>MSQEQLTGSSILAKSLKSLGVDVIFGIVGVPVVEVAEACIAEGIRFIGCRNEQSASFAAGAWGYLNKRPGVCLTVSGPGVVNAISGLYNAQANCWPMILIGGSCETNQIGMGAFQELDQVDACRNYTKFSGKCADLETIPFIVNKAYQVSKAGRPGPTYVDLPADLIQATTSKLPKLPEPFETPYCLPHTKDLSAAIEILKNSKRPLLVVGKGATYSRCENELKALVEEFNVPFLPTPMAKGILPDNHSLNAGSARSLALRKADVIVLLGARLNWMMQFGNRLNPQTKIIHVDISPEEFNINKKIDIGLFGNIPETIELIHQGLKKSGKSYSWIHFKNELQPNIEKNQEKLQKFLTAPLSPLMNHQQALNTVEEVLSKQFNGDYFLVSEGARTMDVTRMLVSSHLPRRRLDAGTLGVMGIGLGYALAGQLTHPDKKVVAIMGDSAFGFSAMEIETAARCKLPLIIIIINNNGIYHGLDDIKSVPSDKLPSFTLMPETRYDLLANSVYGQGFLVKDSTQLQSALQKCFNFDGVSIVNVMIDHRPASEGLYWLTREFSPAGQSKL[4x]

One such enzyme is 2-hydroxyacyl-CoA lyase/synthase (HACL/S), which catalyzes the reversible cleavage of 2-hydroxyacyl-CoA (2hcCoA) into formyl-CoA (fCoA) and an aldehyde or ketone. Originally identified in the mammalian α-oxidation pathway of 3-methyl-branched fatty acids, HACL/S has demonstrated remarkable catalytic reversibility, as it is capable of condensing fCoA with various substrates covering a wide range of aldehydes and ketones with different carbon chain lengths. All the enzymes are tetramers, specifically dimers of dimers (α2), where α2 dimer represents a catalytical unit. The three domains have specific functions: the N-terminal domain binds the pyrimidine of ThDP (PYR), the middle domain has a regulatory function (R) and binds ADP, and the C-terminal domain binds the pyrophosphoryl group (PP) of ThDP.

The α2 interface hosts the ligand binding and catalytic sites that are well-conserved among ThDP-dependent lyases. The overall structural analysis is based on highest resolution structures (1.70 Å TbHACL/S and 1.85 Å CcHACL/S), unless indicated otherwise. The most unique variant is CcHACL/S, showing a clear preference for C3 over C2, and no activity on C1 substrate at all. C1 substrate may be too small to interact with this surface. Curiously, this variant clusters in close proximity with the OXC sub-family, which shows clear preference on C1 and C2 over C3 aldehydes. Comparison of active site structures and ligand binding for CcHACS/L and ApbHACL/S shows relatively small differences but comparison with AcHICL/S shows much larger differences consistent with variations in substrate specificity and kinetic rates. All structures contain well-defined bound ThDP and ADP.>[2x]A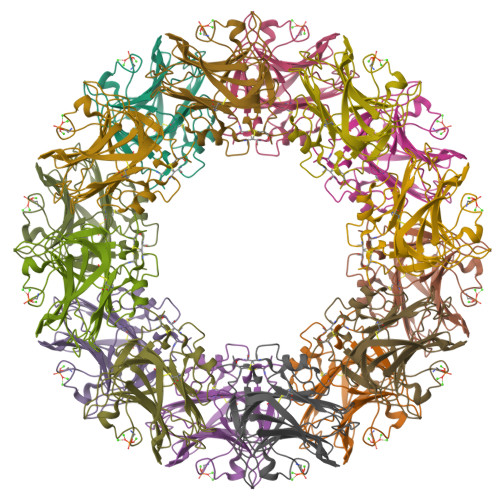VDIRDVKISFPGTQNPKFPHLRFMQTLPAVRQLTVCQRIKPFHRNTGYIFSCATSNQDNQFITSMYVKSDGTLNLGLQVNASSNKYISCPIEIELGQWYHVCHVWSGVDGRMAVYANGSPCGTMENVGKGHQISAGGTVVIGQEQDKIGGGFEEQESWSGELSDLQVWDEALTTHQVSTVASCNGIRPRGNVISWMEDSFVADDGVIVGISHMCSL> MRRTIAALTATPERFSILGTTHPKPKRTGFGRNNKMRSKPSDNVAWYDKGPVEWLPRPVRLTYDHLDQLRDWMMRETLDGKTEEFNRIRDMHREWSQHPLMPVLGDVEPKFPLNLFKQNHRAKRRFL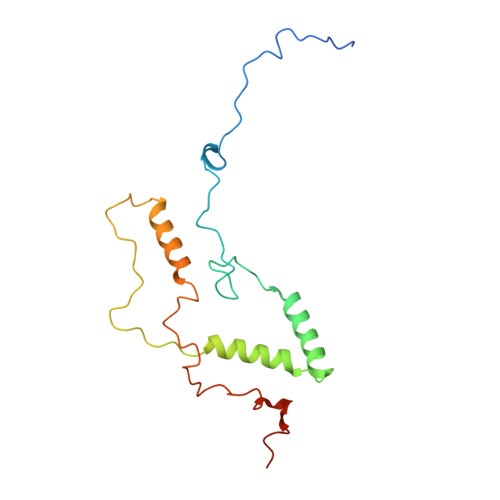VRWHKANTPANWLWMPRGPTVVTPLHHTNPSQYPESWRQMVRKKK> MAQEYTVEQLNHGRKVYDFMRWDYWAFGISGLLLIAAIVIMGVRGFNWGLDFTGGTVIEITLEKPAEIDVMRDALQKAGFEEPMLQNFGSSHDIMVRMPPAEGETGGQVLGSQVLKVINESTNQNAAVKRIEFVGPSVGADLAQTGAMALMAALLSILVYVGFRFEWRLAAGVVIALAHDVIITLGILSLFHIEIDLTIVA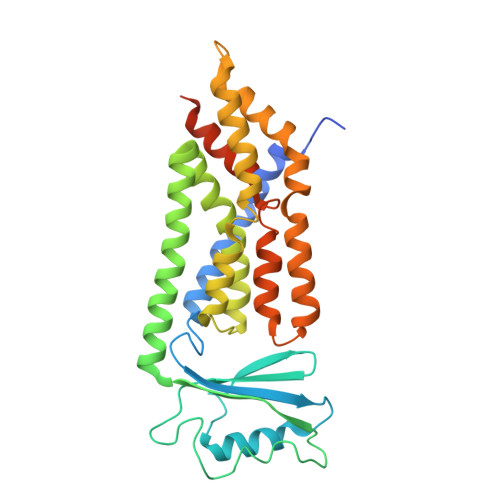SLMSVIGYSLNDSIVVSDRIRENFRKIRRGTPYEIFNVSLTQTLHRTLITSGTTLMVILMLYLFGGPVLEGFSLTMLIGVSIGTASSIYVASALALKLGMKREHMLQQKVEKEGADQPSILP>[2x]MDEFEMIKRNTSEIISEEELREVLKKDEKSAGIGFEPSGKIHLGHYLQIKKMIDLQNAGFDIIIGLADLHAYLNQKGELDEIRKIGDYNKKVFEAMGLKAKYVYGSEEQLDKDYTLNVYRLALKTTLKRARRSMELIAREDENPKVAEVIYPIMQVNSIHYEGV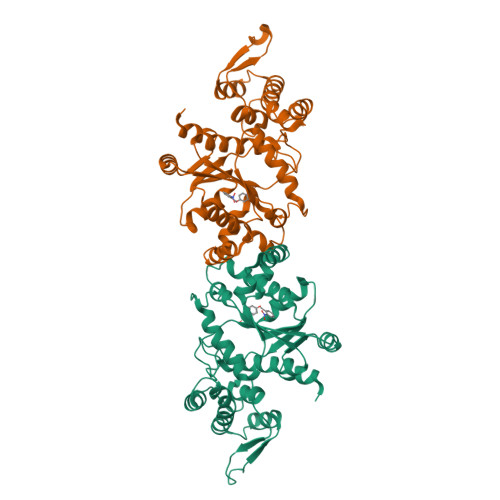DVAVGGMEQRKIHMLARELLPKKVVCIHNPVLTGLDGEGKMSSSKGNFIAVDDSPEEIRAKIKKAYCPAGVVEGNPIMEIAKYFLEYPLTIKRPEKFGGDLTVNSYEELESLFKNKELHPMRLKNAVAEELIKILEPIRKRLSDPENLYFQ>CATGGCCAT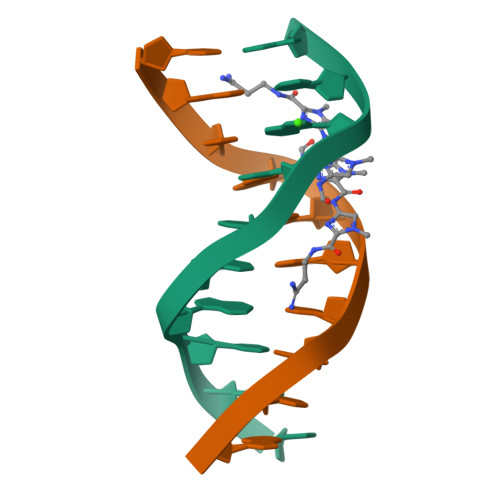G[2x]> MRNFKNDNELLGGNEMPTLYELKQSLGMIGQQLKNKNDELSQKATDPNIDMEDIKQLETEKAGLQQRFNIVERQVQDIEEKEKAKVKDKGEAYQSLSDNEKMVKAKAEFYRHAILPNEFEKPSMEAQRLLHALPTGNDSGGDKLLPKTLSKEIVSEPFAKNQLREKARLTNIKGLEIPRVSYTLDDDDFITDVETAKELKAKGDTVKFTTNKFKVFAAISDTVIHGSDVDLVNWVENALQSGLAAKERKDALAVSPKSGLEHMSFYNGSVKEVEGADMYDAIINALADLHEDYRDNATIYMRYADYVKIISVLSNGTTNFFDTPAEKVFGKPVVFTDAAVKP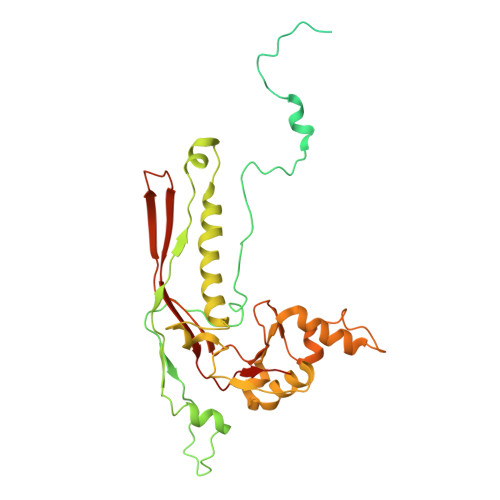IVGDFNYFGINYDGTTYDTDKDVKKGEYLFVLTAWYDQQRTLDSAFRIAKAKENTGPLPS>[16x]FTLIELLIVIAIIAILAAVLIPNLLAARKRANDTVVTAYLNDAVKFQEMYQIDNNSYTSNQAALISLGLKSTPANVTFSIVSASANSYCMIAGHSGGTVWFAATP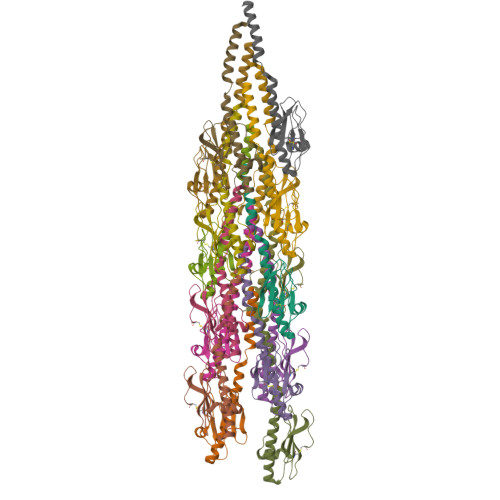DKGVYKTNTAVTSSQPESCP2-acetamido-3-O-[(2S,3S)-2-carboxy-3,4-dihydroxybutan-2-yl]-2-deoxy-alpha-D-glucopyranose 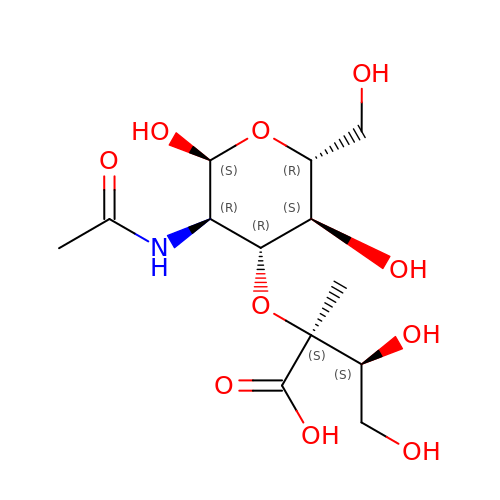| C13 H23 N O10 | NSPVGDAWQINIKU-TXJFNNIZSA-N6,6'-(4-nitro-1H-pyrazole-3,5-diyl)bis(3-bromopyrazolo[1,5-a]pyrimidin-2(1H)-one) | C15 H7 Br2 N9 O4 | 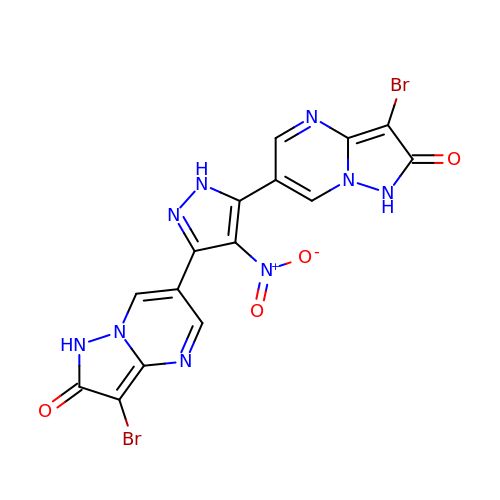ZXUYYFPIPVTPJS-UHFFFAOYSA-N>MAANSTRRPIIAFMSDLGTTDDSVAQCKGLMYSICPDVTVVDVCHSMTPWDVEEGARYIVDLPRFFPEGTVFATTTYPATGTTTRSVAVRIKQAAKGGARGQWAGSGAGFERAEGSYIYIAPNNGLLTTVLEEHGYLEAYEVTSPKVIPEQPEPTFYSREMVAIPSAHLAAGFPLSEVGRPLEDHEIVRFNRPAV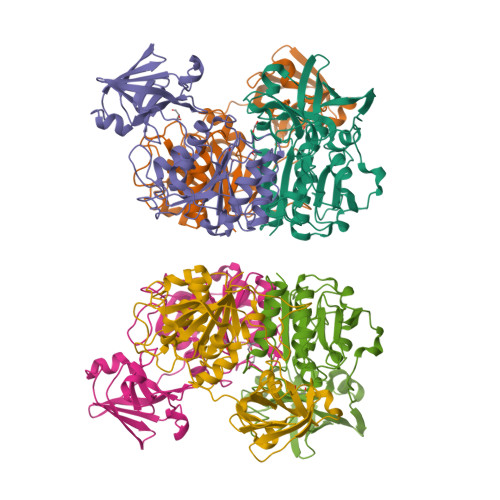EQDGEALVGVVSAIDHPFGNVWTNIHRTDLEKAGIGYGARLRLTLDGVLPFEAPLTPTFADAGEIGNIAIYLNSRGYLSIARNAASLAYPYHLKEGMSARVEAR[6x]> MNWKEFEVFCVT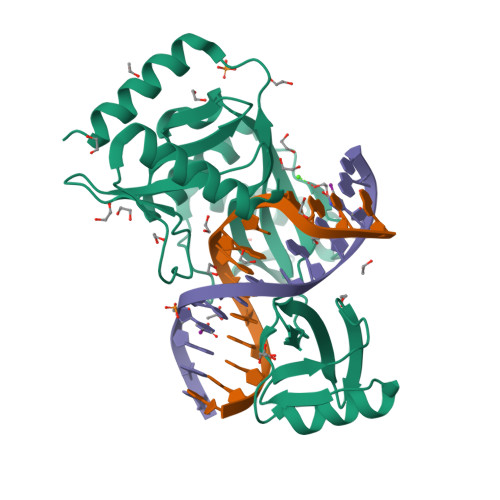YLNKTYGNKFAKKGESDSTTSDILFTGNNPFYIEAKMPHSQCGQFVLIPNRAEYKFDYSPKNKSEINPYTQKIMQFMSENFSEYANLSTKGKIIPLPESVFVNWIKEYYKSKSVKFFITSNGDFIIFPIEHFEHYFNVSCTYRIKKSGSRHLNSKSLPDFKQALDKKGISYTMRGLELHSDENIHDKRISGDDKDFLIKENNGAYHVKILSNTFNANVIFSISLKNNISLFILNEDRKAFEAAISL naphtho[2,1-b]thiophen-1-ylacetic acid | C14 H10 O2 S | 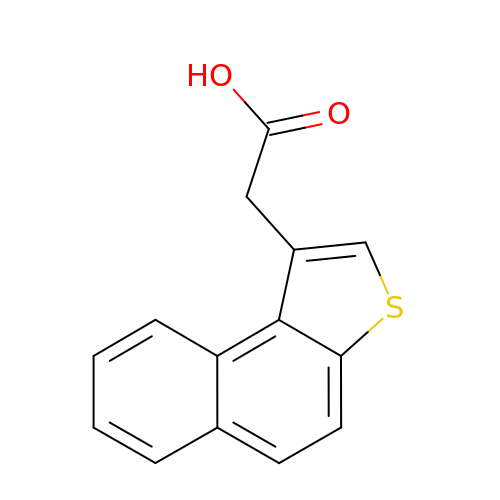SGZIYCCHNHOYKN-UHFFFAOYSA-N>[2x]AQVLRGTVTDFPGFDERADAETLRKAMKGLGTDEESILTLLTSRSNAQRQEISAAFKTLFGRDLLDDLKSELTGKFEKLIVALMKPSRLYDAYELKHALKGAGTNEKVLTEIIASRTPEELRAIKQVYEEEYGSSLEDDVVGDTSGYYQRMLVVLLQANRDPDAGIDEAQV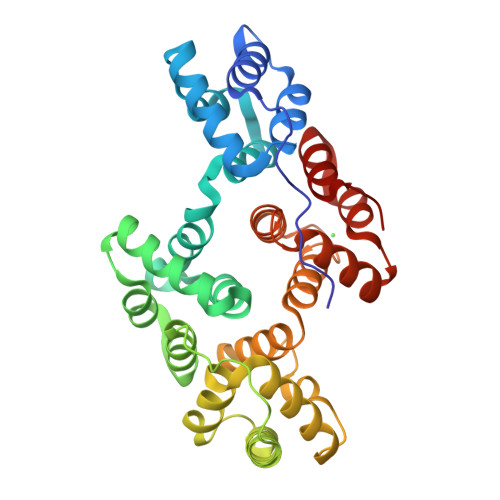EQDAQALFQAGELKWGTDEEKFITIFGTRSVSHLRKVFDKYMTISGFQIEETIDRETSGNLEQLLLAVVKSIRSIPAYLAETLYYAMKGAGTDDHTLIRVMVSRSEIDLFNIRKEFRKNFATSLYSMIKGDTSGDYKKALLLLCGEDD The binding of the plant phytohormone Abscisic acid (ABA) to the family of ABA receptors (PYR/PYL/RCAR) triggers plant responses to abiotic stress. In the resting state, the PYR/PYL receptors are monomers or dimers and display a wide empty ABA binding cavity flanked by two highly conserved loops, named as gate loop and latch loop. To investigate this issue, we have selected as a model SlPYL1 which is a tomato dimeric receptor with known structure that is involved in the induction of stress responsive genes and drought tolerance. Interestingly, the analysis of the structure of SlPYL1 shows that Glu 151 is not involved in the dimerization interface or interacting with ABA; rather, it is located in the latch loop.

To investigate the relevance of this amino acid on the receptor function, we generated a mutated version of SlPYL1 harboring a Glu 151 to Asp substitution (SlPYL1 E151D) at the latch and studied its biochemical properties and compared them with those of the native protein. The overall structures of the apo and ABA bound forms of SlPYL1 E151D are nearly identical to that of WT protein with the differences confined to the area of the mutated residue. In this structure, the apo form showed that Glu 151 and Arg 153 established a salt bridge that blocked the ABA binding pocket while, in the ABA bound form, Glu 151 pointed to the solvent enabling ABA binding and subsequent gate closure (Moreno-Alvero et al., 2017). Instead, the analysis of the apo form of SlPYL1 E151D structure revealed that the shortening of the Glu 151 side chain to Asp disrupts the geometry of the salt bridge with Arg 153, weakening this interaction and favoring the transition to an active receptor. The increased RMSD of the gate and latch loops in the apo forms of SlPYL1 E151D with respect to those of SlPYL1 shows that mutated protein displays higher conformational heterogeneity at these loops. In addition, it reveals that the native structure displays a well-ordered salt bridge between Glu 151 and Arg 153 blocking ABA binding while the mutant protein displays high flexibility for Asp 151 and Arg 153, thus suggesting that the Asp151 mutation might ease the large transition – of the latch for a productive ABA recognition. Indeed, our structural studies corroborated that the mutated latch loop displays higher heterogeneity than the WT, due to the disruption of a salt bridge between Glu 151 and Arg 153 which is capping the entrance to the ABA binding site in the apo form of the receptor. Altogether, the joined analysis of the biochemical and crystallographic data suggests that the weakening of the capping salt bridge in the apo structure of the mutant protein together with the formation of an additional hydrogen bond linking Asp 151 and Thr 110 in the ABA bound structure shift the equilibrium from the apo form to the active form of the mutant receptor.

> MDNKPETSLDNPVHQRSEPGSETGSSLSTITTHHLTVPPGLTPEEFQELSSSIAEFHSYRINPGQCSSLLAQRIHAPVETVWTVVRRFDKPQTYKHFIKSCSVGEDFRMTVGSTRDVTVISGLPAATSTERLDILDDDRHVTGFSIIGGDHRLRNYRSVTTVHGFERDGEIWTVVLESYVVDVPEGNTEEDTRLFADTVVKLNLQKLASVTETLAREAGNGSVNSRDASHRS> TNIYGNGNNVNTDVGANGWAPTVSTGLGDGPVSCTPPTPSPGDTEVPPPRKPFTFPAPPTKSGSRFSKWWEPAAARASESATDSAIEGIDAAGKAASKAITRKLDRPA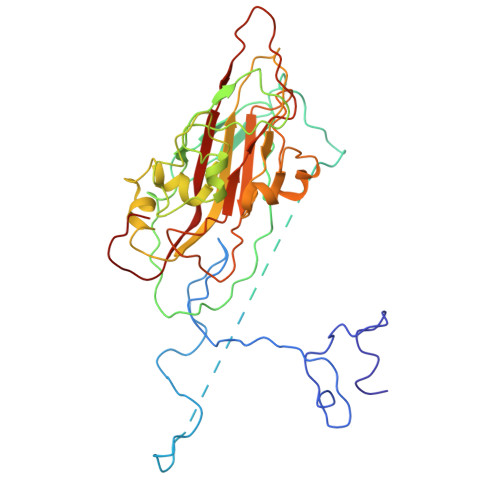APSSTANPQPSLIALNPSATQSGNASILTGSTAPSLLAYPTATPVPLPNPDEPSQPGPSGDRTWLLDTVTWSQEFTRGWNIAGSNGMQWTGLESLIFPVSTDTNWTSTSSPTAYPLPFSFVRAYPDSSWAAMYNTHSMWNCGWRVQVTVNGSQFHAGALILYMVPEATTHAIQTARDNAGFVFPYVILNLYESNTATIEVPYISPTPNTSSGLHAPWTFYLQVLSPLNPPPSLPTSLSCSIYVTPVDSSFHGLRYLAPQ> MMFGRFTERAQKVLALAQEEALRLGHNNIGTEHILLGLVREGEGIAAKALQALGLGSEKIQKEVESLIGRGQEMSQTIHYTPRAKKVIELSMDEARKLGHSYVGTEHILLGLIREGEGVAARVLNNLGVSLNKARQQVLQLLGSNETGSSAAGTNSNANTPTLDSLARDLTAIAKEDSLDPVIGRSKEIQRVIEVLSRRTKNNPVLIGEPGVGKTAIAEGLAQQIINNEVPEILRDKRVMTLDMGTVVAGTKYRGEFEDRLKKVMDEIRQAGNIILFIDALHTLIGAGGAEGAIDASNILKPSLARGELQCIGATTLDEYRKYIEKDAALERRFQPIQVDQPSVDESIQILQGLRDRYEAHHRVSITDDAIEAAVKLSDRYISDRFLPDKAIDLIDEAGSKVRLRSFTTPPNLKELEQKLDEVRKEKDAAVQSQEFEKAASLRDTEQRLREQVEDTKKSWKEKQGQENSEVTVDDIAMVVSSWTGVPVSKIAQTETDKLLNMENILHSRVIGQDEAVVAVAKAVRRARAGLKDPKRPIGSFIFLGPTGVGKTELARALAESIFGDEESMIRIDMSEYMEKHSTSRLVGSPPGYVGYDEGGQLTEKVRRKPYSVVLLD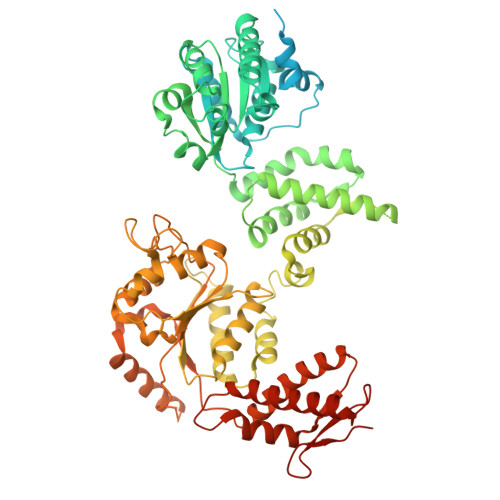AIEKAHPDVFNILLQVLEDGRLTDSKGRTVDFRNTILIMTSNVGASELKRNKYVGFNVQDETQNHKDMKDKVMGELKRAFRPEFINRIDEIIVFHSLEKKHLTEIVSLMSDQLTKRLKEQDLSIELTDAAKAKVAEEGVDLEYGARPLRRAIQKHVEDRLSEELLRGNIHKGQHIVLDVEDGEFVVKTTAKTNLEHHHHHH>MRETRMVYPVFPGETNHYGTLFGGT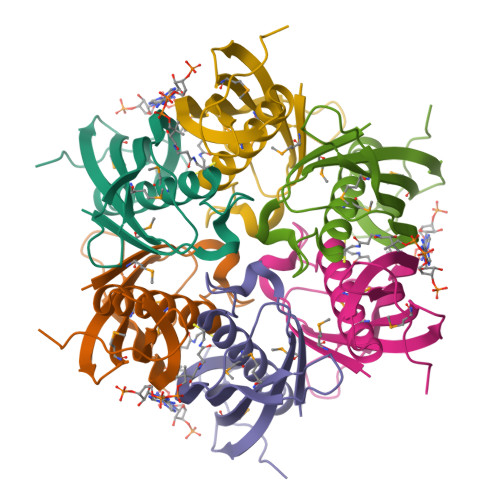VLAWMDQAAFVAATRHARKKVVTVHADAVDFKRPVPLGAIVELVARLKEVGRTSMRVEVEMWVEPVKEGEEAYLAARGGFVLVAVDERGRPSPVPPLEGGEAHAPHGP[2x]>[2x]MADEAQAPPAEGAPPAEGEAPPPAEGAEGAVEGGEAAP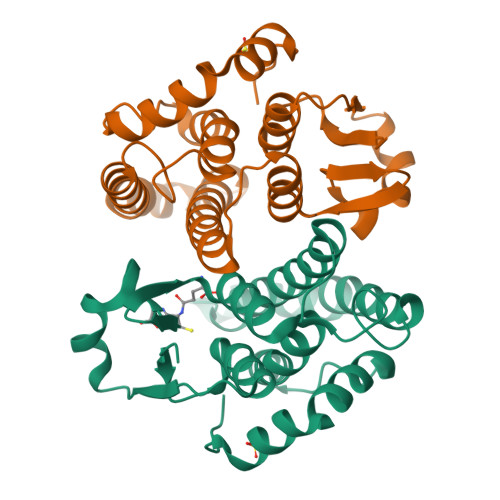PAEPAEPIKHSYTLFYFNVKALAEPLRYLFAYGNQEYEDVRVTRDEWPALKPTMPMGQMPVLEVDGKRVHQSISMARFLAKTVGLCGATPWEDLQIDIVVDTINDFRLKIAVVSYEPEDEIKEKKLVTLNAEVIPFYLEKLEQTVKDNDGHLALGKLTWADVYFAGITDYMNYMVKRDLLEPYPALRGVVDAVNALEPIKAWIEKRPVTEV> MDEFEMIKRNTSEIISEEELREVLKKDEKSAHIGFEPSGKIHLGHYLQIKKMIDLQNAGFDIIISLADLNAYLNQKGELDEIRKIGDYNKKVFEAMGLKAKYVYGSEFGLDKDYTLNVYRLALKTTLKRARRSMELIAREDENPKVAEVIYPIMQVNNSHYFGSDVAVGGMEQRKIHMLARELLPKKVVCIHNPVLTGLDGEGKMSSSKGNFIAVDDSPEEIRAKIKKAYCPAGVVEG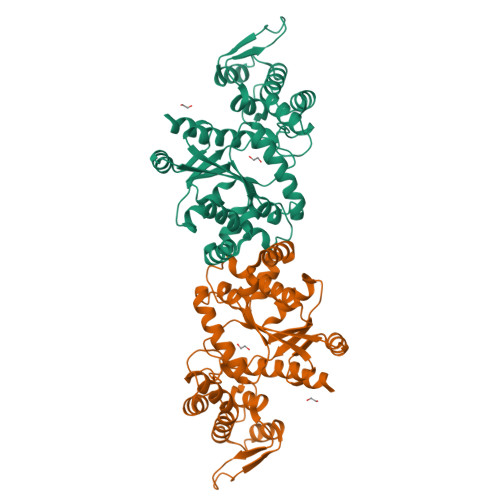NPIMEIAKYFLEYPLTIKRPEKFGGDLTVNSYEELESLFKNKELHPMDLKNAVAEELIKILEPIRKRLLEHHHHHH>[2x]GMNGEAICSALPTIPYHKLADLRYLSRGASGTVSSARHADWRVQVAVKHLHIHTPLLDSERKDVLREAEILHKARFSYILPILGICNEPEFLGIVTEYMPNGSLNELLHRKTEYPDVAWPLRFRILHEIALGVNYLHNMTPPLLHHDLKTQNILLDNEFHVKIADFGLSKWRMMSLSQSRSSKSAPEG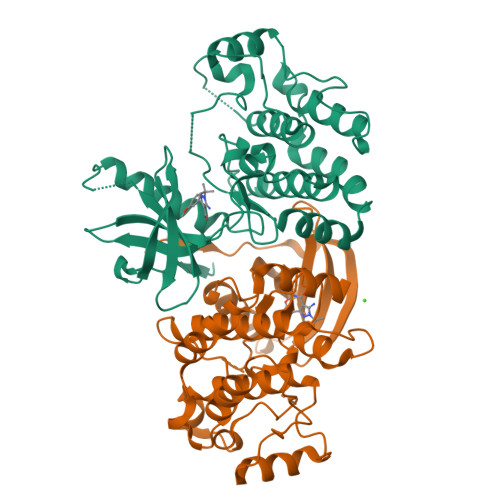GTIIYMPPENYEPGQKSRASIKHDIYSYAVITWEVLSRKQPFEDVTNPLQIMYSVSQGHRPVINEESLPYDIPHRARMISLIESGWAQNPDERPSFLKCLIELEPVLRTFEEITFLEAVIQLK> DI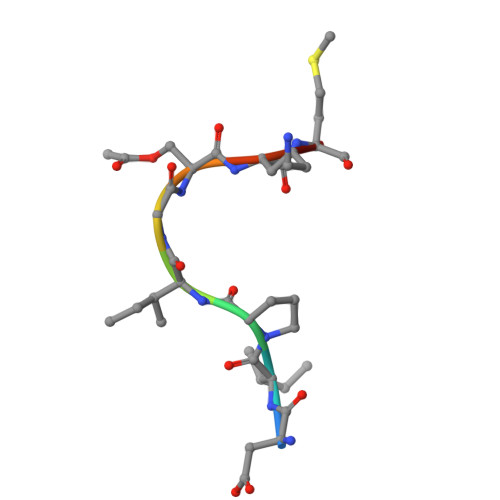PIGSKMT>MTMDEQQSQAVAPVYVGGFLARYDQSPDEAELLLPRDVVEHWLHAQGQGQPSLSVALPLNINHDDTAVVGHVAAMQSVRDGLFCLGCVTSPRFLEIVRRASEKSELVSRGPVSPLQPDKVVEFLSGSYAGLSLSSRRCDDVEQATSLSGSET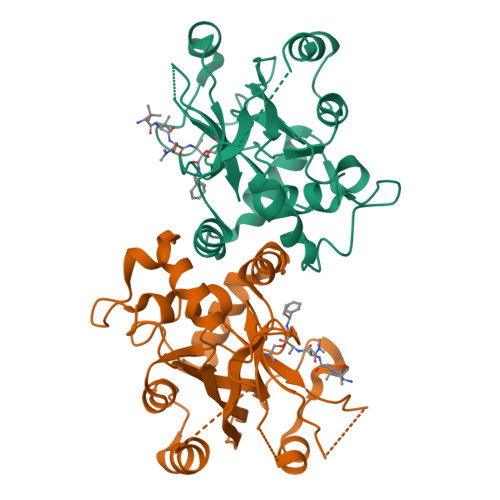TPFKHVALCSVGRRRGTLAVYGRDPEWVTQRFPDLTAADRDGLRAQWQRCGSTAVDASGDPFRSDSYGLLGNYVDALYIRERLPKLRYDKQLVGVTERESYVKA[2x]> MLLNPTKRERKENYSIDNYYKDVLNTGRSSTPSHPRMPKPHVFHSHQLQPPQLQVLYEKERMWTAKKTGYVPTMDDVKAAYGKISDQEEQKEKLELLKLSVNNSQPLTEEEEKMKADWESEGFTNWNKLEFRKFITVSGKYGRNSIQAIARELAPGKTLEEVRAYAKAFWSNIERIEDYEKYLKIIENEEEKIKRVKMQQEALRRKLSEYKNPFFDLKLKHPPSSNNKRTYSEEEDRFILLMLFKYGLDRDDVYELVRDEIRDCPLFELDFYFRSRTPVELARRGNTLLQCLEKEFNAGIVLDDATKDRMKKEDENGKRIREEFADQTANEKENVDGVESKKAKIEDTSNVGTEQLVAEKIPENETTHHHHHHH;> MVAPKPKPAHEQVEPALIPSNWTSVIPLLTSDFKNQYSVISRLKNPNMKPVPYAGDIIKLMAFINKFSSFFHSDLQNLSFQDFEVGLDLYPGDPNGSAAGIVKGPEDTSLLLYPDFMAIKDIVYCQDKMNLLFLSLLDLTFTENFDGKSAKKKGPLTTWENLKSSSKKVFSNPLYRLRLVAREWGYPREWRQQLPSDQDISKPKTALFEQDEQTPVVDPSHPEILTPNIYTWNA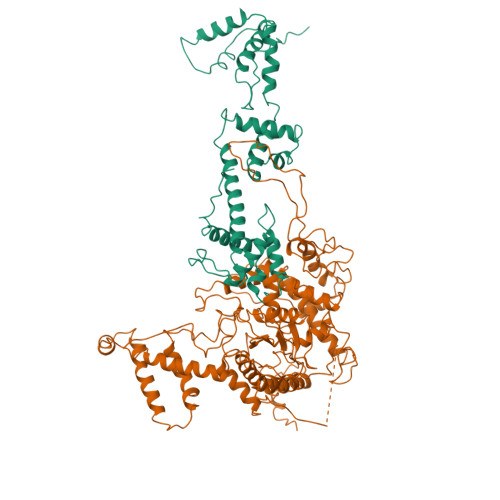NEPLPLESNPLYNREMDKNGILALKPMDRVVLLRALTDWCASHSSAIHDEIYKLTHGKKDPVFGIQTQQVPRYTIEGVDNTINQFKKLCSLIQSRYEIRSKKKHFVKQLKEGKKPDLSRKLEILKEIKAELKNAVKSEKDELLFSLYDKWVPLFEGELPDQPLANPFSERLYKLRLQEFFLGRVPHIGDFYMPRLHSYGDSLEMSTFTDLRNLQALLSKFKNNEYNAFTLFENDGQSMSAQFKLFYHDTPSLAHDVARGRNTSGKVYWYELCHDSATLLEFLEFLDYKIVKPQDEKKEGNEKEKEALNNEAHILEQKSTTDNKPSINTNPLPKDAKYNTARKKLQILKEFLSDYYFILRQFEQMKVQFADMKPGKRQLRRIQRQTVNYNT>MKLAACFLTLLPGFAVAASWTSPGFPAFSEQGTGTFVSHAQLPKGTRPLTLNFDQQCWQPADAIKLNQMLSLQPCSNTPPQWRLFRDGEYTLQIDTRSGTPTLMISIQNAAEPVASLVRECPKWDGLPLTVDVSATFPEGAAVRDYYSQQIAIVKNGQIMLQPAATSNGLLLLERAETDTSAPFDWHNATVYFVLTDRFENGDPSNDQSYGRHKDGMAEIGTFHGGDLRGLTNKLDYLQQLGVNALWISAPFEQIHGWVGGGTKGDFPHYAYHGYYTQDWTNLDANMGNEADLRTLVDSAHQRGIRILFDVVMNHTGYATLADMQEYQFGALYLSGDEVKKSLGERWSDWKPAAGQTWHSFNDYINFSDKTGWDKWWGKNWIRTDIGDYDNPGFDDLTMSLAFLPDIKTESTTASGLPVFYKNKMDTHAKAIDGYTPRDYLTHWLSQWVRDYGIDGFRVDTAKHVELPAWQQLKTEASAALREWKKANPDKALDDKPFWMTGEAWGHGVMQSDYYRHGFDAMINFDYQEQAAKAVDCLAQMDTTWQQMAEKLQGFNVLSYLSSHDTRLFREGGDKAAELLLLAPGAVQIFYGDESSRPFGPTGSDPLQGTRSDMNWQDVSGKSAASVAHWQKISQFRARHPAIGAGKQTTLLLKQGYGFVREHGDDKVLVVWAGQQ[4x]

MalS is an α-amylase that breaks down maltodextrins in the periplasm, hydrolyzing the 1,4-glucosidic bond of amylose and long maltodextrin to release maltohexaose. According to the carbohydrate-active enzymes (CAZy) database, MalS is classified as a member of GH13_19. MalS is an integral component of the maltose utilization pathway in Escherichia coli, crucial to the effective utilization of maltodextrin. MalS degrades linear dextrins by recognizing the substrate at the non-reducing end and preferentially liberating maltohexaose.

The crystal structure of MalS, a periplasmic α-amylase from E.coli strain K12, was determined at a resolution of 2.7 Å. Most of the polypeptide chains had well-defined electron densities, except for residues 1–119, which were not visible in the electron map. MalS consists of four domains: domain A (residues 181–314, 436–645), domain B (residues 315–435), domain C (residues 120–180, 646–676), and the non-visible domain N (residues 1–119). The conventional C-domain of amylase consists of amino acids 120–180 (N-terminal) and 646–676 (C-terminal) in MalS, and the whole domain architecture shows the complete circular permutation of C-A-B-A-C in domain order. The MalS structure has clear disulfide bridges between C121 and C537, located in domains C and A. Based on high electron densities and coordination geometry, we identified two calcium ion positions in the MalS structure. Ca2 is located in domain A, while Ca1 is located between domains A and B. Ca2 is situated at the back of the active center, whereas Ca1 is located near the -3, -4 subsite binding loop. In MalS, Ca1 was located around the -3, -4 subunit binding loop, and thus it stabilized the loop formed by residues 397–406 and participated in substrate binding at the active site. Similar to the catalytic action of common amylases, D460 acts as a nucleophile, E503 as a proton donor, and D565 as a transition state stabilizer. By docking the substrate to MalS, we confirmed that MalS has a binding pocket capable of containing 6 glucose units.> 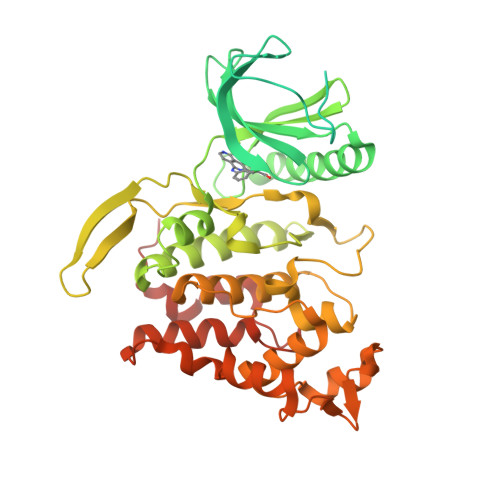MPHPRRYHSSERGSRGSYREHYRSRKHKRRRSRSWSSSSDRTRRRRREDSYHVRSRSSYDDRSSDRRVYDRRYCGSYRRNDYSRDRGDAYYDTDYRHSYEYQRENSSYRSQRSSRRKHRRRRRRSRTFSRSSSQHSSRRAKSVEDDAEGHLIYHVGDWLQERYEIVSTLGEGTFGRVVQCVDHRRGGARVALKIIKNVEKYKEAARLEINVLEKINEKDPDNKNLCVQMFDWFDYHGHMCISFELLGLSTFDFLKDNNYLPYPIHQVRHMAFQLCQAVKFLHDNKLTHTDLKPENILFVNSDYELTYNLEKKRDERSVKSTAVRVVDFGSATFDHEHHSTIVSTRHYRAPEVILELGWSQPCDVWSIGCIIFEYYVGFTLFQTHDNREHLAMMERILGPIPSRMIRKTRKQKYFYRGRLDWDENTSAGRYVRENCKPLRRYLTSEAEEHHQLFDLIESMLEYEPAKRLTLGEALQHPFFARLRAEPPNKLWDSSRDISR>[12x]MNTQATIDTAAVAPLNFDPNAWHHSQMTTLEAIELSRSGGHPYSSPNVPKGFNTVV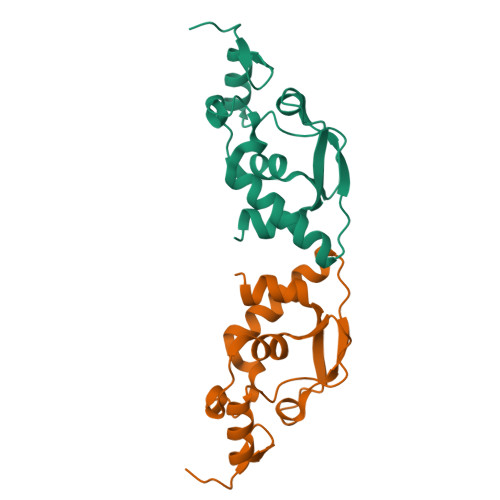GFFFDTYDWYPAAYDDEEGNAMKDRELIQYEDWCAKYARTLGLEVKEVEAPAALKVHGIMALKAYPEALLEIRLIEMP> GMGGSNMKLDFSVAVHSILYLDAHRDSKVASRELAQSLHLNPVMIRNILSVLHKHGYLTGTVGKNGGYQLDLALADMNLGDLYDLTIPPTISYARFITGPSKTDEQADQSPIAANISETLTDLFTVADRQYRAYYHQFTM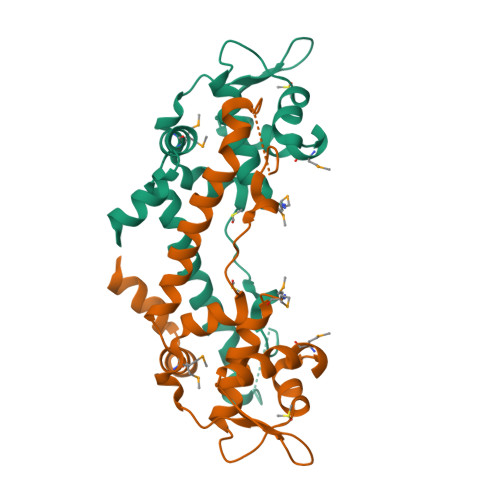ADLQADLNHHGTFLQHEQDSES>[2x]GDADVLVKWSEDLA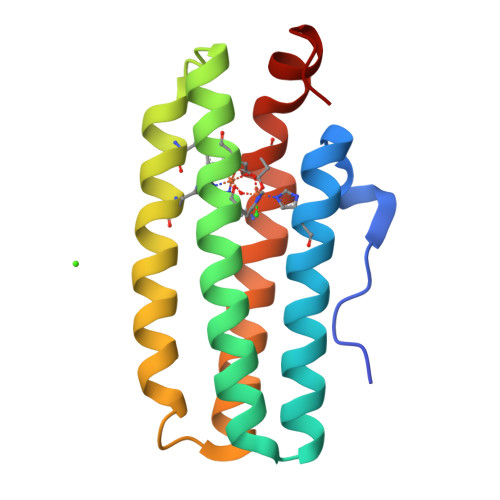NLPSIDTQHKRLVDYINDLYRAARRRDMDKAREVFDALKNYAVEHFGYEERLFADYAYPEATRHKEIHRRFVETVLKWEKQLAAGDPEVVMTTLRGLVDWLVNHIMKEDKKYEAYLRERGVS(2S,5R,6S)-2-benzyl-5,6-bis(4-bromophenyl)-4-methylmorpholin-3-one | C24 H21 Br2 N O2 | 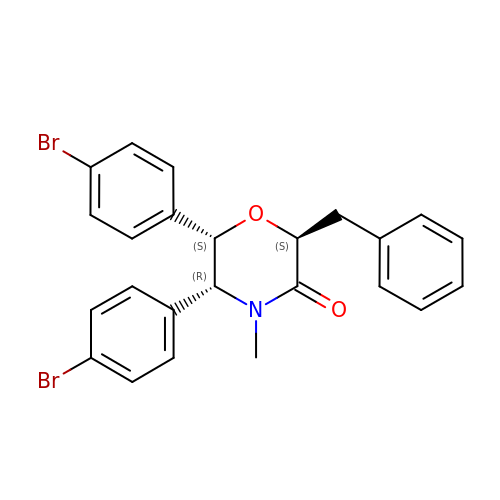YYVYIVSNIAMIER-ZRBLBEILSA-N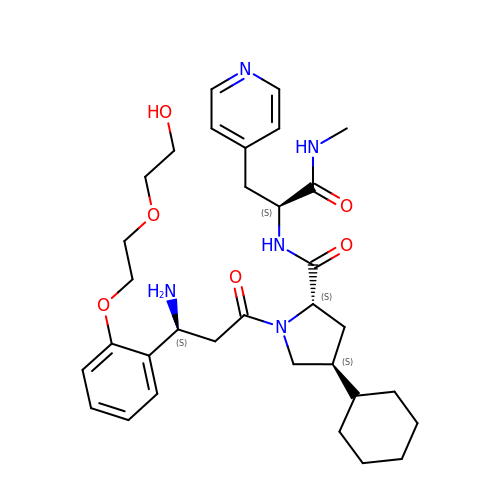(2~{S},4~{S})-1-[(3~{S})-3-azanyl-3-[2-[2-(2-hydroxyethyloxy)ethoxy]phenyl]propanoyl]-4-cyclohexyl-~{N}-[(2~{S})-1-(methylamino)-1-oxidanylidene-3-pyridin-4-yl-propan-2-yl]pyrrolidine-2-carboxamide | C33 H47 N5 O6 | GDZUYXCMNWYMAG-ZIZDPRJYSA-N>GAMAMHPMLNIAVRAARKAGNLIAKNYETPDAVEASQKGSNDFVTNVDKAAEAVIIDTIRKSYPQHTIITEESGELEGTDQDVQWVIDPLDGTTNFIKRLPHFAVSIAVRIKGRTEVAVVYDPMRNELFTATRGQGAQLNGYRLRGSTARDLDGTILATGFPFKAKQYATTYINIVGKLFNECADFRRTGSAALDLAYVAAGRVDGFFEIGLRPWDFAAGELLVREAGGIVSDFTGGHNYMLTGNIVAGNPRVVKAMLANMRDELSDALKR[2x];> GAMDNKPADDLLNLEGVDRDLAFKLAARGVCTLEDLAEQGIDDLADIEGLTDEKAGALIMAARNICWFGDEA

Ribosomal RNA synthesis in Escherichia coli involves a transcription complex, in which RNA polymerase is modified by a signal element on the transcript, Nus factors A, B, E and G, ribosomal protein S4 and inositol mono-phosphatase SuhB. This complex is resistant to ρ-dependent termination and facilitates ribosomal RNA folding, maturation and subunit assembly. We show that SuhB directly binds the RNA signal element and the C-terminal AR2 domain of NusA, and we delineate the atomic basis of the latter interaction by macromolecular crystallography. The SuhB monomers are folded as an alternating stack of three pairs of α helices (helix pairs I–III) and two β sheets.

To begin elucidating the structural basis underlying the transcriptional functions of SuhB, we determined a crystal structure of a SuhB-NusAAR2 complex at 1.65 Å resolution. An asymmetric unit of the crystals contained two SuhB molecules and a single copy of NusAAR2. The AR2 domain formed a dual helix-hairpin-helix motif with four α helices and one 310 helix (order α1-α2-α3–310-α4), as observed before in other molecular contexts. The SuhB monomers formed a near-C2-symmetrical dimer that closely resembled the previously observed dimer of an isolated SuhBR184A variant (rmsd 0.66 Å for 491 pairs of common Cα atoms). In the SuhB-NusAAR2 crystal, two symmetry-related copies of NusAAR2 were bound laterally at equivalent surfaces of the two SuhB subunits of the dimer, i.e. below one exposed edge of sheet I and along the exposed lateral face of helix pair II, sheet II and helix pair III of SuhB. However, one of the NusAAR2 copies associated with one SuhB subunit via a flat surface formed by its C-terminal α3–310-α4 portion (interaction mode 1), while the other AR2 domain bound the second SuhB subunit via an edge formed by its α1, α3 and α4 elements (interaction mode 2). Interaction modes 1 and 2 bury about 650 Å2 and about 500 Å2 of combined surface area, respectively, showing that interaction mode 1 encompasses a more extended interface between SuhB and NusAAR2. Moreover, superimposing the AR2 domain of a αCTD–NusAAR2 complex on the AR2 domains in the SuhB-NusAAR2 crystal structure revealed that SuhB bound in interaction mode 1 would preclude αCTD–AR2 interactions, while interaction mode 2 would allow formation of a ternary SuhB–NusAAR2–αCTD complex. Thus, only interaction mode 1 can explain the mutually exclusive binding of SuhB and αCTD to NusAAR2 we observed. The analyses were again consistent with interaction mode 1 representing the relevant complex, as SuhB mutations affecting interaction mode 1 led to a reduction of more than three orders of magnitude in the affinity to AR2 (Kd = 141 μM for SuhBKL251/254AA-AR2), while a SuhB mutation affecting interaction mode 2 only had a mild effect (∼4.5-fold reduction in affinity; Kd = 435 nM for SuhBK108A-AR2).> GVNSVAARVTELTGREVAAVAERGHSHRWHLYRVELADGTPLFVKALPDDAPALDGL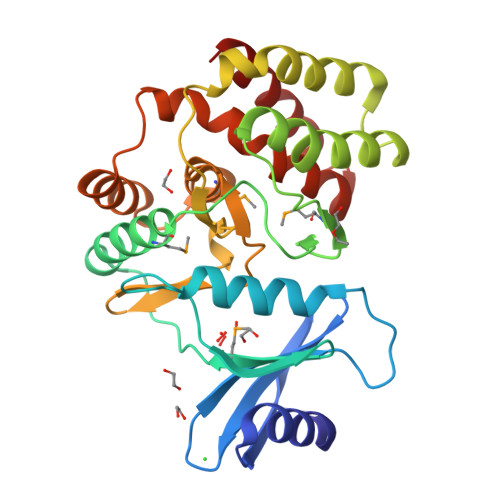FRAEALGLDWLGRSFGSPVPQVAGWDDRTLAMEWVDERPPTPEAAERFGHQLAAMHLAGAESFGATWDGYIGPLPMDNTPRSTWPEFYAEQRILPYLRRAADRGALTPGDVRLVEKVLDALDHLAGDPEPPARIHGDLWNGNVLWQDDGAVVIDPAAHGGHREADLAMLALFGLPYLDRVRDAYNEVAPLAEGWRARIPLHQLHPLLVHVCLFGAAYRTTLVDTARAALRA> QAQITGRPEWIWLALGTALMGLGTLYFLVKGMGVSDPDAKKFYAITTLVPAIAFTMYLSMLLGYGLTMVPFGGEQNPIYWARYADWLFTTPLLLLDLALLVDADQGTILALVGADGIMIGTGLVGALTKVYSYRFVWWAISTAAMLYILYVLFFGFTSKAESMRPEVASTFKVLRNVTVVLWSAYPVVWLIGSEGAGIVPLNIETLLFMVLDVSAKVGFGLILLRSRAIFGEAEAPEPSAGDGAAATSD

Membrane proteins localize in the lipid bilayer of biomembranes and play a variety of important functions such as transport of various substances between the inside and outside of the cell, signal transduction, energy synthesis, and cell adhesion. We developed amphipathic compounds, phospholipid mimics and detergents bearing multiple halogen substitutions on aromatic rings for de novo phasing and revealing lipid-protein interactions. Serial femtosecond crystallography (SFX) is a new data measurement technique of X-ray crystallography, which takes advantage of the ultra-high beam brilliance, femtosecond pulse duration and high spatial coherence of XFEL. Because femtosecond XFEL diffraction in SFX is completed on a shorter timescale than the process of radiation damage and photoreduction, this technique captures the damage-free structure of samples.

The structural properties of HAD16 mimic a phosphatidylcholine structure. HAD16 can be used as a tool for analyzing lipid-membrane protein interactions. Microcrystals of bacteriorhodopsin obtained by the bicelle method were mixed with HAD16 and then SFX data were collected at SACLA (Supplementary Materials Section S7). Although two heavy atom sites were located by the SIR, SIRAS or SAD method, auto-tracing was not possible even with all 18,069 lattices obtained. This is most likely because of the smaller isomorphous and anomalous signal from HAD16, which contains only one I atom and one Br atom per molecule instead of three I atoms in HAD13a, as well as only one HAD16 molecule in the asymmetric unit when compared with two HAD13a molecules. The HAD16 molecule adopting alternative conformations binds to an interface region among three symmetry-related bacteriorhodopsin molecules. The long alkyl tail of HAD16 interacts with the hydrophobic transmembrane surface. The choline and phosphate group face the bulk solvent. The aromatic ring in the head group ring is stabilized by π–π stacking with Y26 and hydrophobic interactions of I/Br atoms with L22, G23, V127, and L221 from a bacteriorhodopsin molecule and W80 from a neighboring molecule. Because a lipid or detergent molecule is located in the corresponding site of the native bacteriorhodopsin structure, we concluded that HAD16 binds to the same site by partially replacing the lipid or detergent. Thus, we modeled lipid/detergent-derived alkyl chains and HAD16 together using partial occupancies.> GMEIHFEKVTSDNRKAVENLQVFAEQQAFIESMAENLKESDQFPEWESAGIYD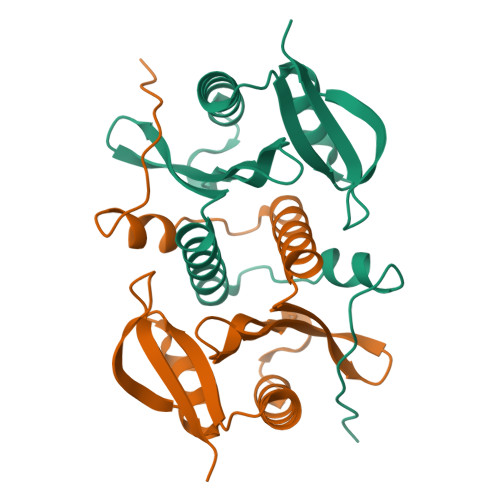GNQLIGYAMYGRWQDGRVWLDRFLIDQRFQGQGYGKAACRLLMLKLIEKYQTNKLYLSVYDTNSSAIRLYQQLGFVFNGELDTNGERVMEWTHQNK>[2x]MKTVTVKNLIIGEGMPKIIVSLMGRDINSVKAEALAYREATFDILEWRVDHFMDIASTQSVLTAARVIRDAMPDIPLLFTFRSAKEGGEQTITTQHYLTLNRAAIDSGLVDMIDLELFTGDADVKATVDYAHAHNVYVVMSNHDFHQTPSAEEMVLRLRKMQALGADIPKIAVMPQSKHDVLTLLTATLEMQQHYADRPVITMS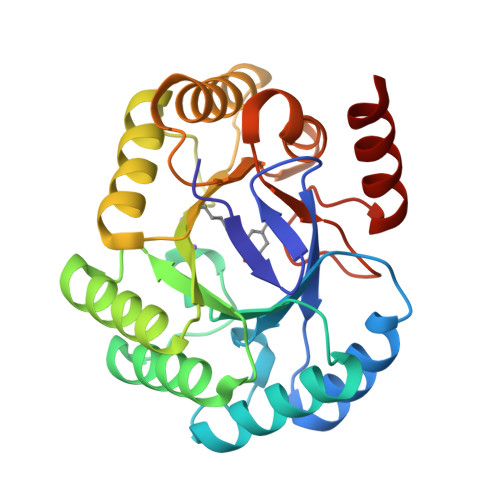MAKEGVISRLAGEVFGSAATFGAVKQASAPGQIAVNDLRSVLMILHNA>[4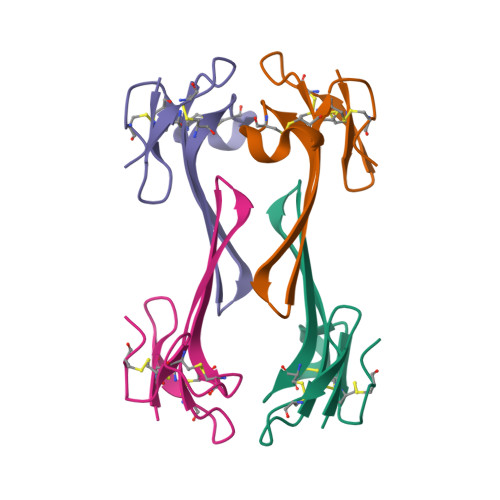x]LKCYQHGKVVTCHRDMKFCYHNTGMPFRNLKLILQGCSSSCSETENNKCCSTDRCNK>[4x]M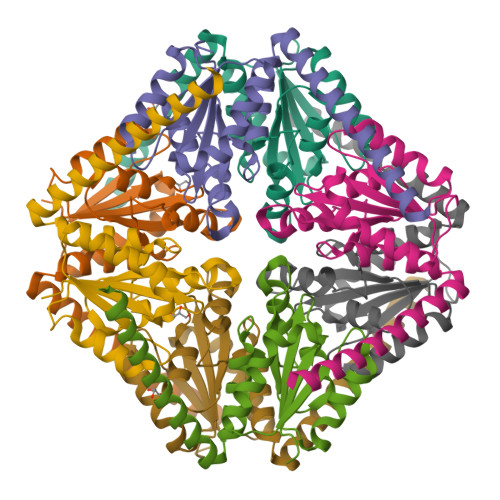TPAGERPRVGVIMGSDSDWPVMADAAAALAEFDIPAEVRVVSAHRTPEAMFSYARGAAARGLEVIIAGAGGAAHLPGMVAAATPLPVIGVPVPLGRLDGLDSLLSIVQMPAGVPVATVSIGGAGNAGLLAVRMLGAANPQLRARIVAFQDRLADVVAAKDAELQRLAGKLTRD>GGEGTDAIQALIQAYFTAWNTNAPE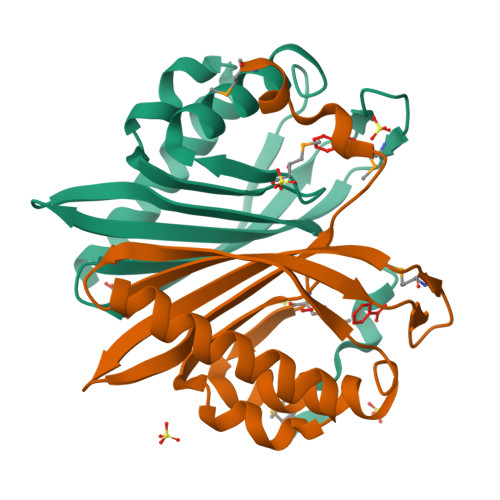RFAEIFWPDGSWVNVVGMHWRGRDQIVFAHTAFLKTIFKDCKQELVTIEARTIAPGSALAVVTLIQDAYVTPDGRQMPRAHDRLTLLAVEREGVWRFIHGHNTIVNPDAANNDPVLRMKPA[2x]>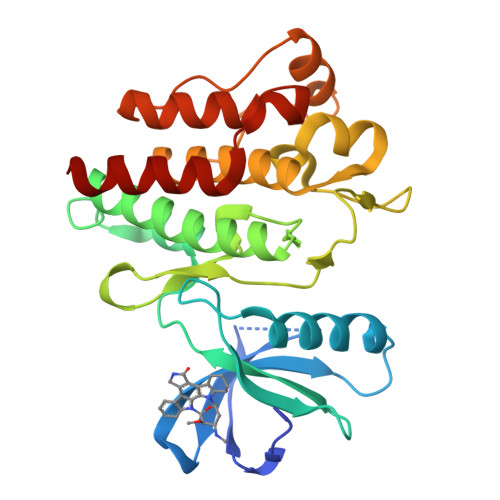VSPNYDKWEMERTDITMKHKLGGGQYGEVYEGVWKKYSLTVAVKTLKEDTMEVEEFLKEAAVMKEIKHPNLVQLLGVCTREPPFYIITEFMTYGNLLDYLRECNRQEVNAVVLLYMATQISSAMEYLEKKNFIHRDLAARNCLVGENHLVKVADFGLSRLMTGDTYTAHAGAKFPIKWTAPESLAYNKFSIKSDVWAFGVLLWEIATYGMSPYPGIDLSQVYELLEKDYRMERPEGCPEKVYELMRACWQWNPSDRPSFAEIHQAFETMFQES[3x]> MMSIAQVRSAGSAGNFYTDKDNYYVLGSMGERWAGRGAEQLGLQGSVDKDVFTRLLEGRLPDGADLSRMQDGSNRHRPGYDLTFSAPKSVSMMAMLGGDKRLIDAHNQAVDFAVRQVEALASTRVMTDGQSETVLTGNLVMALFNHDTSRDQEPQLHTHAVVANVTQHNGEWKTLSSDKVGKTGFIENVYANQIAFGRLYREKLKEQVEAL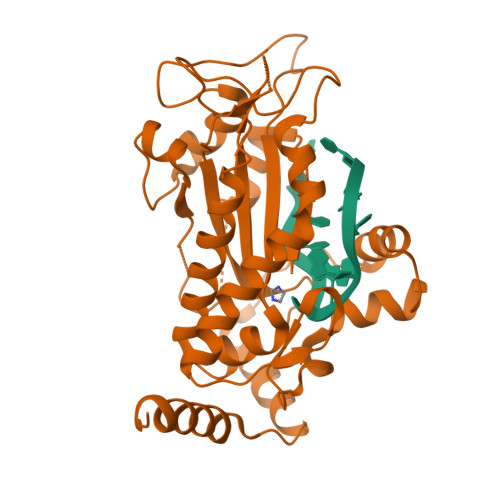GYETEVVGKHGMWEMPGVPVEAFSGRSQTIREAVGEDASLKSRDVAALDTRKSKQHVDPEIKMAEWMQTLKETGFDIRAYRDAADQRADLRTLTPGPASQDGPDVQQAVTQAIAGLSER>[2x]SGIREVILCKDQDGKIGLRLKSIDNGIFVQLVQANSPASLVGLRFGDQVLQINGENCAGW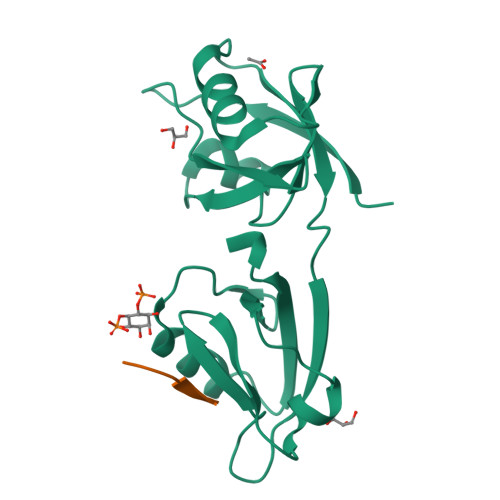SSDKAHKVLKQAFGEKITMTIRDRPFERTITMHKDSTGHVGFIFKNGKITSIVKDSSAARNGLLTEHNICEINGQNVIGLKDSQIADILSTSGTVVTITIMPAFIF;>[2x]KGETAV> MENTENSVDSKSIKNLEPKIIHGSESMDSGISLDNSYKMDYPEMGLCIIINNKNFHKSTGMTSRSGTDVDAANLRETFRNLKYE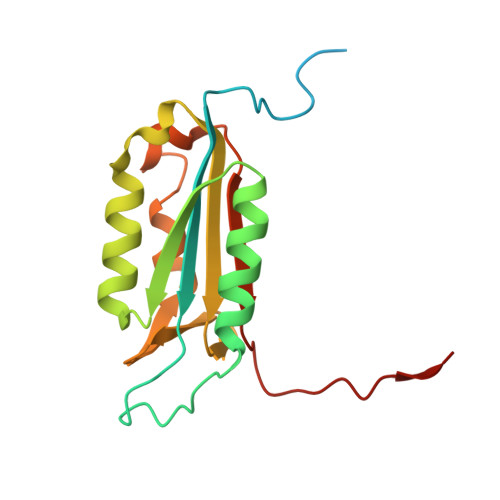VRNKNDLTREEIVELMRDVSKEDHSKRSSFVCVLLSHGEEGIIFGTNGPVDLKKITNFFRGDRCRSLTGKPKLFIIQAARGTELDCGIETD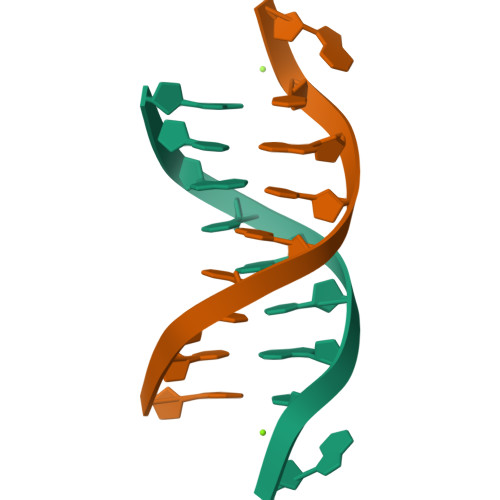> GCGTACGCG>HYPEFSWDTVPIAFHFGKSQGLLTKEEAEFVATRSNFICLEKGHATRTHGTTEAGIEAEARQLKNLNPKMKVIFYWNTFLDYSMFAAHKEYAKHPQWWLRTTTGELDRKKGQLMRYDLSNAEFRNWWTNVAAKAVVDGTCDGVFMDAFPQIASQANRKLWGDEKFEAIQQGLQDIIQETRQKIGDDKLIVYNGIRSTPDWSAGFDFAEYTDAAMIEHFGHFQSASKETMLRDILEMQRAAKAGKIVVLKGWAGFTFIDDQAMRKPLTQKRRVAKDSLKFPLACFLAGAQENCYFIYNWGYRMENGCLEWYP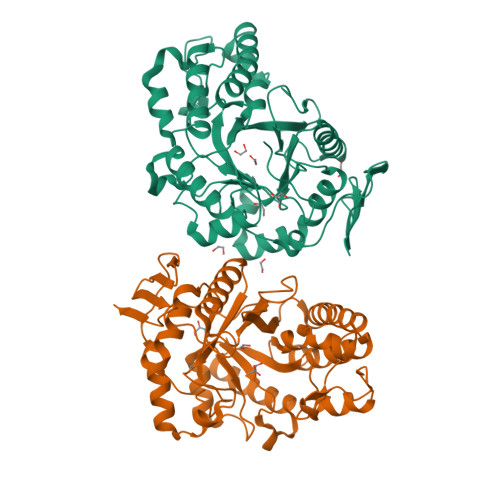EFDKPLGKPVGEMVRDGWKLSREYKHASVRVDLESKEAEIRWR[2x]> GSRDNLLFGDEIITNGFHSCESDEEDRASHASSSDWTPRPRIGP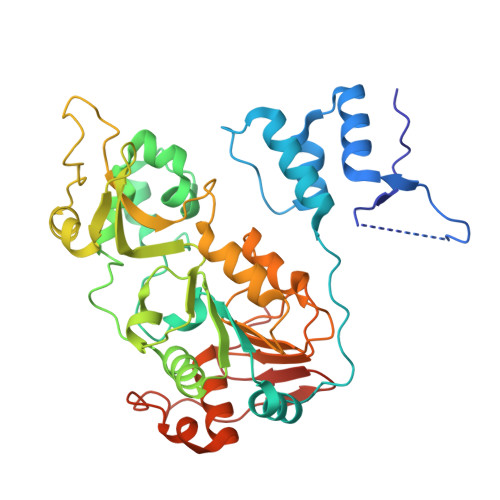YTFVQQHLMIGTDPRTILKDLLPETIPPPELDDMTLWQIVINILSEPPKRKKRKDINTIEDAVKLLQESKKIIVLTGAGVSVSSGIPDFRSRDGIYARLAVDFPDLPDPQAMFDIEYFRKDPRPFFKFAKEIYPGQFQPSLCHKFIALSDKEGKLLRNYTQNIDTLEQVAGIQRIIQCHGSFATASCLICKYKVDCEAVRGDIFNQVVPRCPRCPADEPLAIMKPEIVFFGENLPEQFHRAMKYDKDEVDLLIVIGSSLKVRPVALIPSSIPHEVPQILINREPLPHLHFDVELLGDCDVIINELCHRLGGEYAKLSSNPVKLSEITEQYLFLPPNRYIFHGAEVYSDSEDDV>[4x]GSHMSQATSQPINFQVQKDGSSEKSHMDDYMQHPGKVIKQNNKYYFQTVLNNASFWKEYKFYNANNQELATTVVNDNKKADTRTINVAVE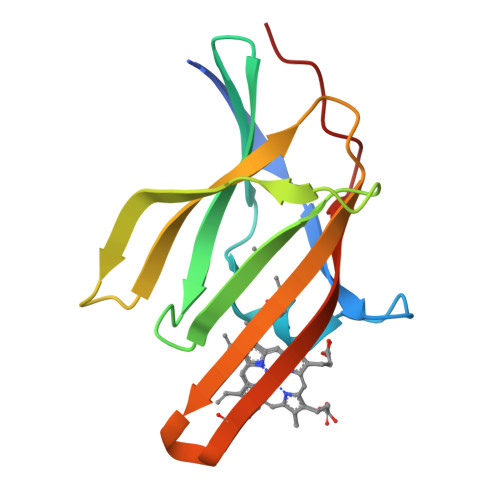PGYKSLTTKVHIVVPQINYNHRYTTHLEFEKAIPTLA> MLTGVIEGFYGRDWRRDERATVMDWIAAAGMNTYIYGPKDDVHVRARWRVPYDAAGLARLTELRDAAAARGMVFYVSLAPCLDVTYSDPQDRAALLARVDQLARAGLRNLVLLFDDIPSVLPEADRHRFDSFAEAQADLSNMVLRHLRGAGHVVFCPTEYCGRMAGGDPRGSAYLQRLGSTLDPAIDIFWTGPEIVSEEIVAAHLAAVGEVLRRRPVIWDNFHANDYDIRRVFAGPLGGRSRDILPLVAGWITNPNNEAEANFPAIHTTGAYLADPDYAPERAIAAAVAAWQPRFRLAFGDGAVPSDLVALLCDLFWQPFALG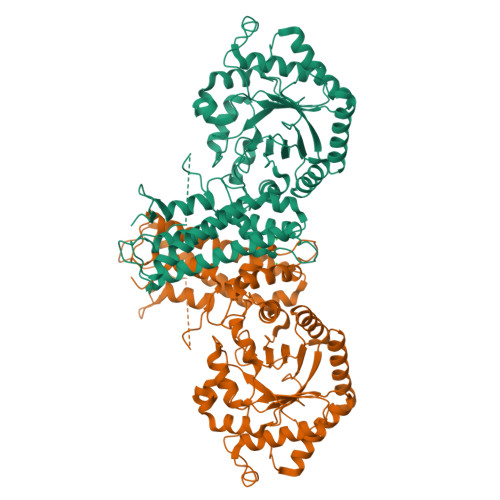PETTRILSALRAALTVPRPDPSDPAWRAALEDLRDLKRRINKLFTLMTEIENRDLFHTFHNYLWEAQEEVGHLVAYCDWLDEAPPPGAVFPATDRIHNFYRRGFGVAVQDILQRDRQGRYHHGV>SNASKGMALRSVGGMVIESPRNETEHWLLETVGRQAQQAGIGMPTVAIYDSADINAFATGAKRDDSLVAVSTGLLHNMTRDEAEAVLAHEVSH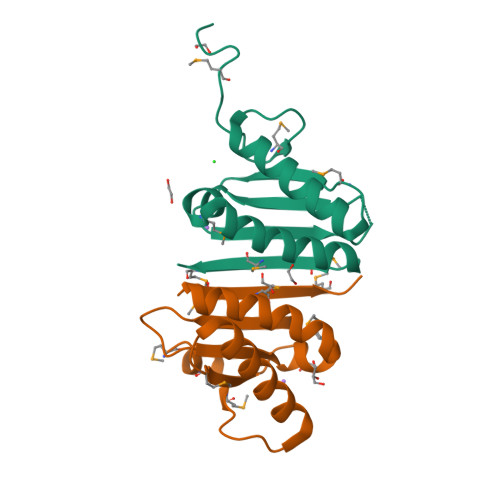IANGDMVTMTLMQG[2x]> SPSVEACGYSDRVAQLTVGNSTITTQEAANIVLSYGEWPGYCPSTDATAVDKPTRPD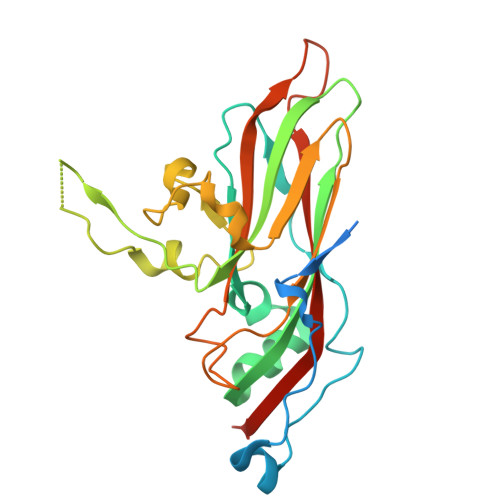VSVNRFYTLSTKSWKTESTGWYWKFPDVLNDTGVFGQNAQFHYLYRSGFCMHVQCNASKFHQGALLVVVIPEFVVAASSPATKPNGQGLYPDFAHTNPGKEGQVFRDPYVLDAGIPLSQALVFPHQWINLRTNNCATIIMPYVNALPFDSALNHSNFGLAVIPISPLKYCNGATTEVPITLTIAPLNSEFSGLRQAIKQ> MTGTNPLYRGSMVALSLKISIGNVVKTM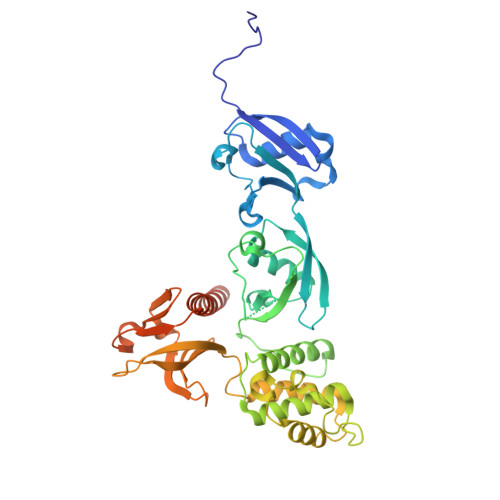QFEPSTMVYDACRMIRERIPEALAGPPNDFGLFLSDDDPKKGIWLEAGKALDYYMLRNGDTMEYRKKQRPLKIRMLDGTVKTIMVDDSKTVTDMLMTICARIGITNHDEYSLVRELMEEKKDELNWLDHGRTLREQGVEEHETLLLRRKFFYSDQNVDSRDPVQLNLLYVQARDDILNGSHPVSFDKACEFAGFQCQIQFGPHNEQKHKAGFLDLKDFLPKEYVKQKGERKIFQAHKNCGQMSEIEAKVRYVKLARSLKTYGVSFFLVKEKMKGKNKLVPRLLGITKECVMRVDEKTKEVIQEWSLTNIKRWAASPKSFTLDFGDYQDGYYSVQTTEGEQIAQLIAGYIDIILKKKKSKDHFGLEGDEESTMLEDSVSPKKST> SRMRAVLHLEHKRYFQNHGHILFEGLAPVSDCKQLEAELKLFLKEVAVVKDRH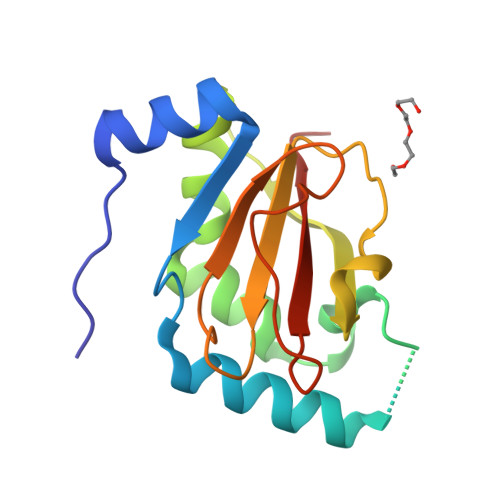LQRWRENVHRTLPGVQMIVKRVRLDHLAAELTHRSRVALVRDLWVQKQEEILFDDCDCSVLLCLSGEKAGWGLFFSGEYPQDVFDWGAGDTAIILRFSSAGFPN> MGLK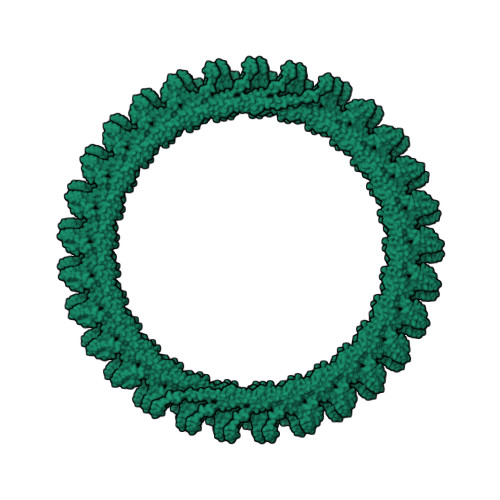KKLFPRKKGKEKANLITNAKVHIHKLNLVNRNYTKRAEISRKNAKIALRRGEKTRAKNFLIQYKSYNAKIDRSNNIRSKIERQIQAIEEGQLISQTGSIFEGIRDELKYIATEASPAKVAEIAEDSDVYVSEIEEAADILAGDPEIDLGIDVTDELNQLETELLLSQGGTMPDAPSDDLQYIPEYGDELEEEVESKTKEKVQAEIEKLRKELES>[6x]SSEMKTEDELRVRHLEEENRGIVVLGINRAYGKNSLSKNLIKMLSKAVDALKSDKKVRTIIIRSEVPGIFCAGADLKERAKMSSSEVGPFVSKIRAVINDIANLPVP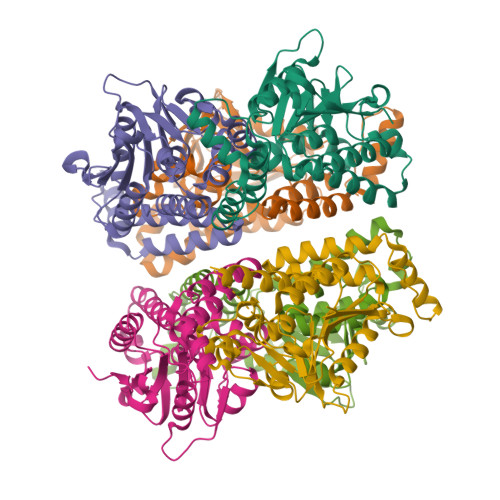TIAAIDGLALGGGLELALACDIRVAASSAKMGLVETKLAIIPGGGGTQRLPRAIGMSLAKELIFSARVLDGKEAKAVGLISHVLEQNQEGDAAYRKALDLAREFLPQGPVAMRVAKLAINQGMEVDLVTGLAIEEACYAQTIPTKDRLEGLLAFKEKRPPRYKGE> MGHHHHHHMAQKPVDNITQIIGGTPVVKLRNVVDDNAADVYVKLEYQNPGGSVKDRIALAMIEKAEREGKIKPGDTIVEPTSGNTGIGLAFVCAAKGYKAVFTMPETMSQERRNLLKAYGAELVLTPGSEAMKGAIKKAKELKEEHGYFEPQQFENPANPEVHELTTGPELLQQFEGKTIDAFLAGVGTGGTLSGVGKVLKKEYPNIEIVAIE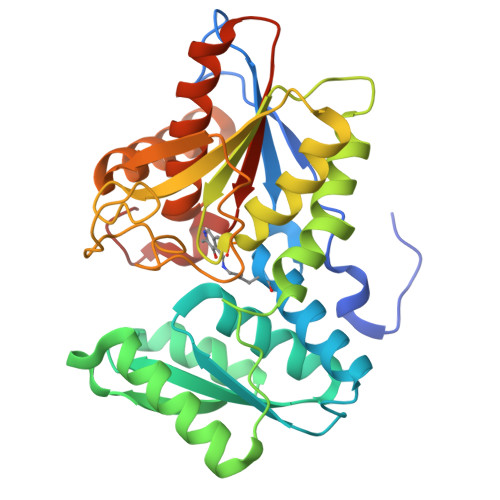PEASPVLSGGEPGPHKLQGLGAGFIPGTLNTEIYDSIIKVGNDTAMEMSRRVAKEEGILAGISSGAAIYAAIQKAKELGKGKTVVTVLPSNGERYLSTPLYSFDD>SMPPPPEVSPVTGNPVSPHYIHSSTLHFQDVNGRSLVLRGVNLSGSAKHPNNQPSHIREGFWETAEAGKGDFINKPLNLDDGSADLHLARLKAWGYNLLRYVFTWESLEHAGPKEYDYAYMDYIIAVLRKCKEWGFRVFMDPHQDVWSRFTGGSGAPLWTLYACGIDPYHLTATAAAYLHCEWPSAESPKP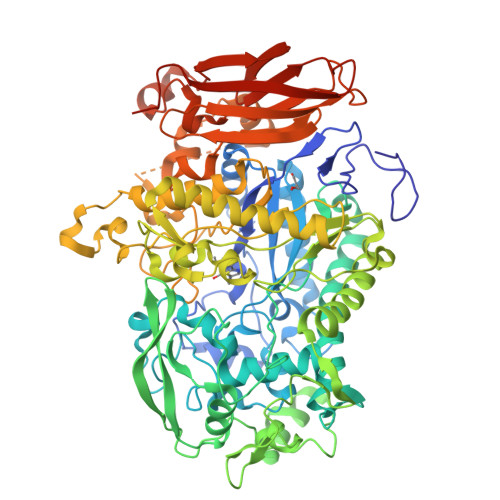QDFPAMIWGTNYTHLANQTIWTFFFAGKTYAPKCIIDGKNIQDFLQDHFIDAVGELAKRIAEEAGDLLDECVIGWDSINEPGEGLIGCKDLAVIPAEQQLKKGPSPTPIEGMRLGMGEAQDVQAWNFGPMGPYRGSRQTIDPKGVKLWLSKEDDVKRGSGKWGWTRGKEWALGTCIWAHHGVWEIATSTLLRPDYFSTLPTNPGHQVDFVDDFWALHWLAYSSRIRLHHPESIHFIQAPVLRQPPKLPESFLKGRACSSPHFYDGLTLMTKHWNWFNADAIGVIRKKYWSIVQAVRIGEGPIRKMIQGELAVLKQDTIDILGNYPTLVGEIGIPYDMDDKKAYGYVDGGRGEGDYSSQQKAMDCSMNACDGPNCLNYAIWNYVPDNVHEWGDNWNGEDLSLWSVDDKEQESYHDSPRSDTPNFSTNSNSLTNSSATLTVPMSGASKLRPSPSVIDSGDFSPTLILDGSRAVAAFCRPYPVATVGIPERIDFDITSTKFKYAVRVRADDIANEQVYTEIYLPFVHYAASLNASYSSFAQLSLDVTIVASHGRVEIQGQTLRWWYPVPGTGEEVYTIEVQRNGGALRRDLGYVQQGNFLDVCPECVIA[4x]> GHMPLLSASIVSAPVVTSETYVDIPGLYLDVAKAGIRDGKLQVILNVPTPYATGNNFPGIYFAIATNQGVVADGCFTYSSKVPESTGRMPFTLVATIDVGSGVTFVKGQWKSVRGSAMHIDSYASLSAIWGTAA

BC2L-C is a new type of lectin from Burkholderia cenocepacia that binds (mammalian) fucosides at the N-terminal domain and (bacterial) mannosides at the C-terminal domain. BC2L-C presents a double carbohydrate specificity, with a Man-specific carbohydrate recognition domain (CRD) in the C-terminal domain and a Fuc-specific CRD in the trimeric N-terminal domain. Thus, BC2L-C can contribute to adhesion and colonization by simultaneously binding bacterial mannosides and human fucosides, and it has been dubbed a superlectin. We have recently described the rational design and synthesis of a first group of antagonists of Burkholderia cenocepacia BC2L-C lectin, a candidate target for AAT against this pathogen, which is associated with fatal pulmonary infections of cystic fibrosis patients.

In order to understand the atomic details of the interaction, the structure of BC2L-C-Nt was solved in complex with compound 3. The electron density revealed, without ambiguity, that ligand 3 displaced all of the blood group oligosaccharide. Only the hexagonal crystal form was refined at 1.55 Å, with one protomer in the asymmetric unit and the trimer forms, by applying the 3-fold crystallographic symmetry. All the interactions at the fucose moieties are equivalent to the one described in previous structures, with the binding site located in a shallow groove at the interface between protomers. Binding interactions involve direct H-bonds of all the fucoside oxygens with Thr74, Arg85*, Thr83* and Arg111 (* amino acid from neighboring protomer). Two structural waters mediate H-bonds between O2 and O3 hydroxyls and Ser 82*, Tyr58 and Tyr75, and hydrophobic contacts are made with Tyr48* ring and the C6 methyl. On the aglycone part, only the two nitrogen atoms are involved in hydrogen bonds mediated through water molecules. The terminal amine is interacting with the main chain oxygen of Asp118* via two water molecules, the main chain nitrogen of Tyr120* and OD1 atom of Asp70 via one water molecule, and with the OD2 atom of Asp70 via two water molecules. The amine in compound 3 occupies the position of a water molecule in the complex of 2, which was involved in mediating the interaction between the amine and the side chain of Asp70. The affinities measured corroborate the NMR-STD results, showing that 3, with a KD of 159 µM, is only 3 times less potent than the H-type 1 tetrasaccharide, and is over one order of magnitude more potent than α-methyl fucoside.> STDNAETGVIEAGNTDTDFSGELAAPGSNHTNVKFLFDRSRLLNVIKVLEKDAV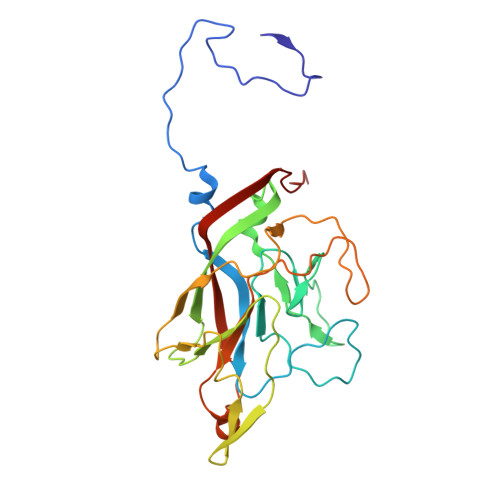FPRPFPTATGTQQDDGYFCLLTPRPTVASRPATRFGLYVSPSDSGVLANTSLDFNFYSLACFTYFRSDLEVTVVSLEPDLEFAVGWFPSGSEYQASSFVYDQLHVPYHFTGRTPRAFASKGGKVSFVLPWNSVSSVLPVRWGGASKLSSATRGLPAHADWGTIYAFIPRPNEKKSTAVKHVAVYIRYKNARAWCPSMLPFRSYK> GAMEAVNMNVEKPTVYHCKVFQFKNLQNPKIRFKLKMNSKELSLKGLCLRIRDDGPGIIIVVGNEKSCKFYENL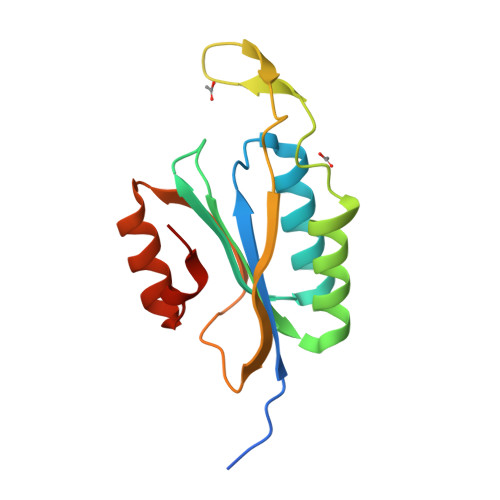VMKRIKWNEDFELHTNTGDIKMDMHNNSISKTWEGYLQDCKFKGWFMKVCNDQDSLLRTLGQFDSEHFYSPVQT>[2x]GGSMATNENLPEIMTKLWDSKAQGEQEELHLLKGSDCNLTIDITEKCLRLAQRSAYQLHTETSATKRIQKFFLLGSLNINKDDRVIINIDRFDPGRIIDRKEGNKSLHVPTAVIPGDVIIPLSMQLACLGSEGVSPFSISEYYDAFQTLTKNLKLSCDSVDIKDMLSLKIHATYYVDSDEISINVTSGVVVPSALITAVPILPVSIVPTALARSLSGPLHLSNFQDTQKSGYVAINNSHNLLLVLDSDPKLSSIPLVGIWVDGVISIHHPYVWSACMRYLYSQRLTNKIRDGSTGFILVLYTQTRPKPEFWECSFSGKSDKFLYCQASDDIFMEKVAKTRNEYMRLQLVPNEFGENLYFQ

Here we demonstrate that CEP85 is essential for faithful centriole duplication through a direct interaction with the previously uncharacterised N-terminal domain of STIL, a key factor involved in the early steps of centriole formation. Subsequently, through its C-terminal PB3, PLK4 interacts with STIL and phosphorylates it, enabling STIL to recruit SASS6 to the site of procentriole assembly.

The NTD of STIL revealed a global structural similarity to the N-terminal domain of the autophagy-related protein ATG7, a protein–protein interaction domain that forms binary complexes with Atg10 and Atg356. It is composed of two subdomains that are structurally akin to each other suggesting that this domain might have evolved via a domain duplication and fusion event. The common structural core of both subdomains consists of a six-stranded open β-barrel capped at the top and on one side with α-helices, a fold that resembles the so-called MPN/JAB1/PAD-1/JAMM domain, as observed, for example, in eIF3f. The STIL NTD subdomain 1 is structurally more akin to MPN domains than the subdomain 2 and this similarity extends to the position and length of the capping helix and the presence of a crossover hairpin-loop, connecting strands 4 and 7. Interestingly, we found that these capping helices and their vicinity in both STIL NTD subdomains define the most conserved patches on their surface making them prime candidates for a role in protein–protein interactions, in this instance binding to CEP85 cc4. The structure of the STIL NTD showed the presence of two conserved patches on its surface. Thus, it is possible that the STIL NTD binds other factors, as yet undiscovered, that might compete or synergise with CEP85 binding or be involved in CEP85 independent functions.>GPGSMGDVNWDTLQKAAVAARANSYAPYSNFPVGVAGFVNDGRLITGVNVENASYGLALCAECSMISALYATGGGRLVAVYCVDGNGDSLMPCGRCRQLLYEHGGPELKIMTPKGVQTMAQLLPQAFNPQERIFGN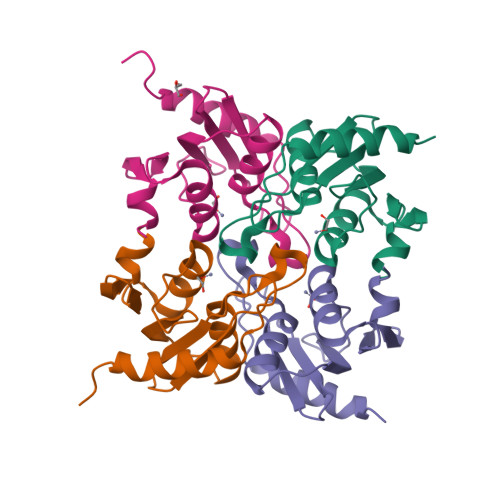DE[4x]(2~{S},3~{S},4~{R})-2-[[4-[4-(2-ethoxyethoxy)phenyl]-1,2,3-triazol-1-yl]methyl]pyrrolidine-3,4-diol 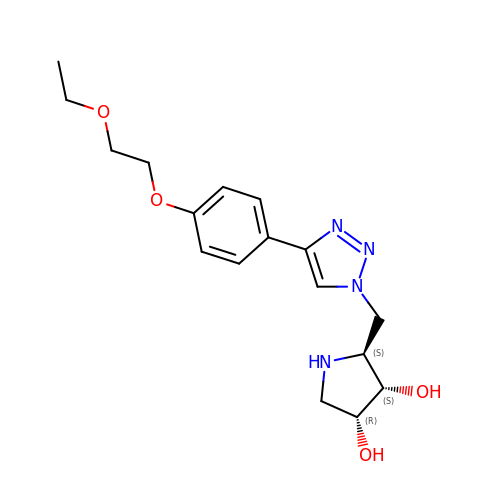| C17 H24 N4 O4 | NXQXJVDZMOHAEW-BBWFWOEESA-N>[2x]GSGSHVTLPFYPKSPQSKDLIKEAILDNDFMKNLELSQIQEIVDCMYPVEYGKDSCIIKEGDVGSLVYVMEDGKVEVTKEGVKLCTMGPGKVFGELAILYNCTRTATVKTLVNVKLWAIDRQCFQTIMMRTGLIKHTEY

The cGMP-dependent protein kinases (PKG) belong to the family of serine/threonine kinases and are one of the major intracellular receptors for cGMP. Next, two cyclic-nucleotide binding domains (CNBD-A and CNBD-B) are followed by the catalytic domain. Binding of cGMP to the CNBDs is thought to induce a conformational change that activates the kinase by removing the autoinhibitory domain from the catalytic cleft, leaving the catalytic domain free to phosphorylate downstream substrates. To understand the overall architecture of the cGMP-binding domain and the molecular features required for cGMP binding, we determined crystal structures of the CNBD-A of human PKG I bound to cGMP, cAMP or in the absence of bound nucleotide.

Each cGMP binding site in the PKG Iβ:cGMP crystal shows a clear electron density for cGMP bound in a syn configuration, as previously predicted by mutation and other studies. The cGMP-binding site is comprised of three parts: the short P-helix together with conserved glutamate and arginine residues at the PBC which captures the sugar phosphate (Site 1); a key residue, Thr193 at the end of PBC that bridges the cyclic phosphate to the guanine ring (Site 2); and the β5-strand that provides a unique docking site for the guanine ring (Site 3). The exposed backbone amides of Gly182, Glu183, Leu184 and Ala185 of the P-helix together with the guanidinium group of Arg192, captures the cyclic phosphate through several hydrogen bonds and electrostatic interactions. In addition, the hydroxyl group of Thr193 interacts with the equatorial OP1 of cGMP, bridging the phosphate moiety to the guanine ring of cGMP. While Leu172 makes a nonpolar contact with a carbonyl group at the C6 position of the guanine ring, Cys173 interacts with the unprotonated N7 of the guanine ring through an extended hydrogen bond. The crystallographic dimer is formed mainly by the bound cGMP, the helical tip of the PBC, and the αB-helix from one molecule (molecule B) fitting onto similar regions on the second molecule (molecule A). While cGMP in molecule B (cGMP:B) is partially exposed to solvent, cGMP in molecule A (cGMP:A) is wedged between the two molecules and participates in crystallographic packing of the two molecules. Superimposition with the B and H forms of the PKA RIα CNBD-A reveals that the PKG Iβ CNBD-A:cGMP complex is in a conformation that more closely resembles the H-form of RIα, not the B-form. The CNBD-A bound with syn-configured cGMP shows the lowest B-factors, implying that interaction with the guanine ring is strongest at site 3 compared to other structures.ethyl 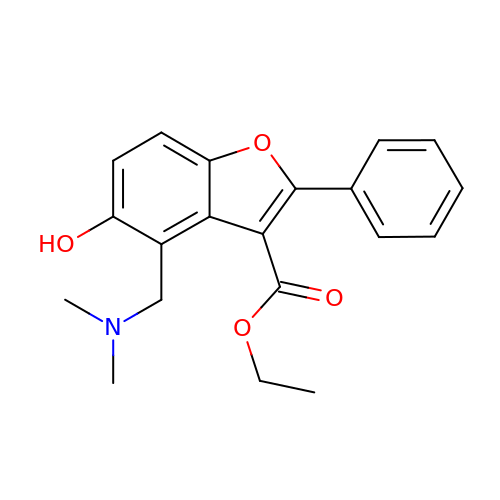4-[(dimethylamino)methyl]-5-hydroxy-2-phenyl-1-benzofuran-3-carboxylate | C20 H21 N O4 | JXUHSUSCLWIKEW-UHFFFAOYSA-N> MQVLHVCSEMFPLLKTGGLADVIGALPAAQIADGVDARVLLPAFPDIRRGVTDAQVVSRRDTFAGHITLLFGHYNGVGIYLIDAPHLYDRPGSPYHDTNLFAYTDNVLRFALLGWVGAEMASGLDPFWRPDVVHAHDWHAGLAPAYLAARGRPAKSVFTVHNLAYQGMFYAHHMNDIQLPWSFFNIHGLEFNGQISFLKAGLYYADHITAVSPTYAREITEPQFAYGMEGLLQQRHREGRLSGVLNGVDEKIWSPETDLLLASRYTRDTLEDKAENKRQLQIAMGLKVDDKVPLFAVVSRLTSQKGLDLVLEALPGLLEQGGQLALLGAGDPVLQEGFLAAAAEYPGQVGVQIGYHEAFSHRIM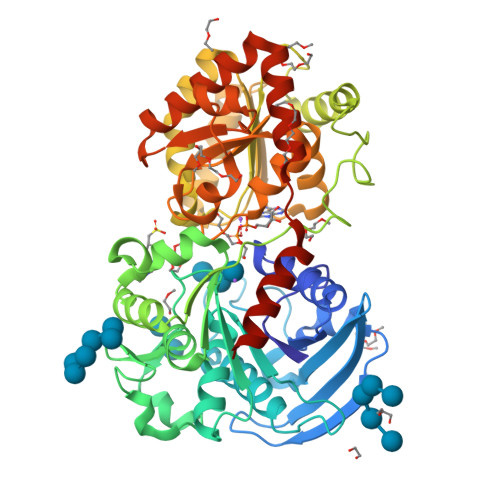GGADVILVPSRFAPCGLTQLYGLKYGTLPLVRRTGGLADTVSDCSLENLADGVASGFVFEDSNAWSLLRAIRRAFVLWSRPSLWRFVQRQAMAMDFSWQVAAKSYRELYYRLKLEHHHHHH>GSDWVIPPINLPENSRGPFPQELVRIRSGRDKNLSLRYSVTGPGADQPPTGIFIINPISGQLSVTKPLDRELIARF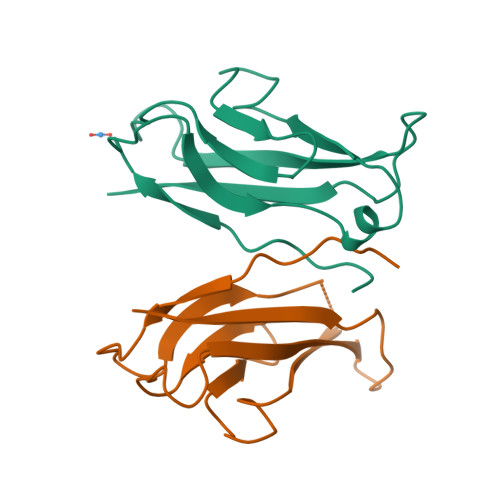HLRAHAVDINGNQVENPIDIVINVIDMNDNRPEF[2x]>[2x]MQRREFLKLSALGVGAMALRGSGPAKALKAPWYAQEVKSVYQICEGCFWRCGIVAHAVGNRVYKVEGYEANPKSRGRLCPRGQGAP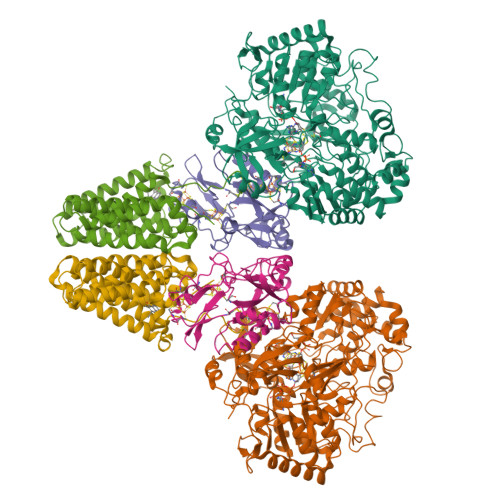QTTYDPDRLKRPLIRVEGSQRGEGKYRVATWEEALDHIAKKMLEIREKYGPEAIAFFGHGTGDYWFVDFLPAAWGSPNAAKPSVSLCTAPREVASQWVFGRPIGGHEPIDWENARYIVLIGHHIGEDTHNTQLQDFALALKNGAKVVVVDPRFSTAAAKAHRWLPIKPGTDTALLLAWIHVLIYEDLYDKEYVAKYTVGFEELKAHVKDFTPEWAEKHTEIPAQVIREVAREMAAHKPRAVLPPTRHNVWYGDDTYRVMALLYVNVLLGNYGRPGGFYIAQSPYLEKYPLPPLPLEPAAGGCSGPSGGDHEPEGFKPRADKGKFFARSTAIQELIEPMITGEPYPIKGLFAYGINLFHSIPNVPRTKEALKNLDLYVAIDVLPQEHVMWADVILPEATYLERYDDFVLVAHKTPFIQLRTPAHEPLFDTKPGWWIARELGLRLGLEQYFPWKTIEEYLETRLQSLGLDLETMKGMGTLVQRGKPWLEDWEKEGRLPFGTASGKIELYCQRFKEAGHQPLPVFTPPEEPPEGFYRLLYGRSPVHTFARTQNNWVLMEMDPENEVWIHKEEAKRLGLKEGDYVMLVNQDGVKEGPVRVKPTARIRKDCVYIVHGFGHKAPLMRLAHGRGASDNYLQTRYKLDPISGGAGLRVNFVRLEKAERPRLPSLTGLAKRPFDERRM;>[2x]MPRYAMAIDLSLCVGCAACAVACKMENEVPPGVFNLWIREREVGEYPNLVVEFRPEQCLHCENPPCVPVCPTGASYQTKDGLVLVDPKKCIACGACIAACPYDARYLHPAGYVSKCTFCAHRLEKGKVPACVETCPTYCRTFGDLEDPESPVAKALKAAERVDVLRPEQGTRPKLFYLNAPSKKGLTRESEVHHG;>[2x]MAEFYGLPNAQEFWHWTNALHFVLVGLAGGVALLAALLHLKGDAEARRYTLYALMLIALDLFILWAESPARFRFTHIWLFLSFHPTSPIWWGAWGLGLGFLTGGLLYLGKGSQRALAWALLVFSLVALSYPGLALAVNLNRPLWNGLMAGLFPLTALVLALGLAALLKSPWALFPLRVLAGASLLLALLYPLTLPPEARGHLLEEAGFWYGLFLLLGLGTFWQERLAPWAGLLAAAGLRALLVLAGQWQGLGL>[2x]GPLGSMSLTPLCEDLPQFLQNYLPNAG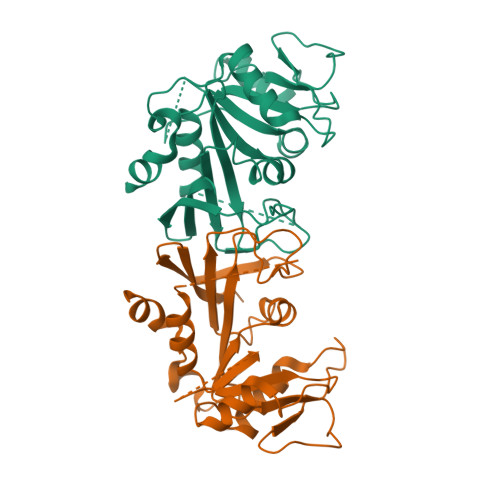QTENTIVPFVTLTYAQSLDARVSRGPGVRTTISHPETKTMTHYLRHHHDGILVGSGTVLADNPGLNCKWGPDPAANSPRPIIIDTKQKWRFDGSKMQELFIKRQGKPPIVVVTSEPIIKEQHVDYAICPINDTTKLVDWKKLFEILKEEFNIRSVMVEGGANVINQLLLRSDIVNSLIITIGSTFLGSSGTEVSPPQTVNLKDMSWWKGITDVVLCARLADD>[2x]GDTKEQRILRYVQ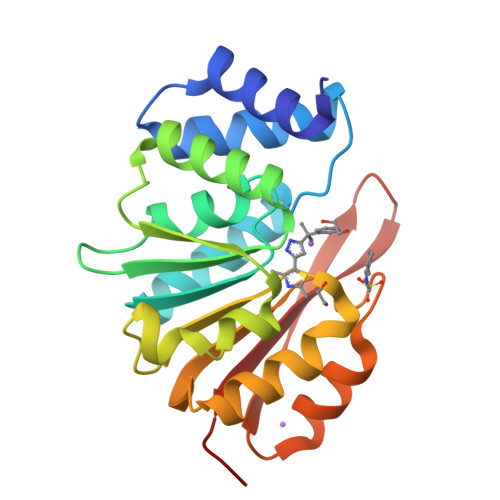QNAKPGDPQSVLEAIDTYCTQKEWAMNVGDAKGQIMDAVIREYSPSLVLELGAYCGYSAVRMARLLQPGARLLTMEINPDCAAITQQMLNFAGLQDKVTILNGASQDLIPQLKKKYDVDTLDMVFLDHWKDRYLPDTLLLEECGLLRKGTVLLADNVIVPGTPDFLAYVRGSSSFECTHYSSYLEYMKVVDGLEKAIYQGPS>AQVINTFDGVADYLQTYHKLPDNYITKSEAQALGWVASKGNLADVAPGKSIGGDIFSNREGKLPGKSGRTWREADINYTSGFRNSDRILYSSDWLIYKTTDHYQTFTKIR[3x];>[3x]KKAVINGEQIRSI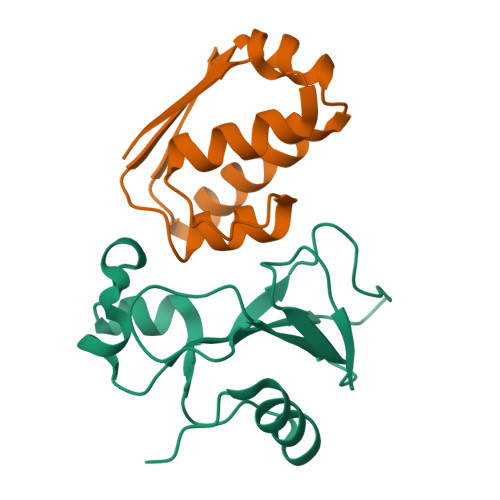SDLHQTLKKELALPEYYGENLDALWDALTGWVEYPLVLEWRQFEQSKQLTENGAESVLQVFREAKAEGADITIILS>[2x]MSDLETVAKFLAESVIASTAKTSERNLRQLETQD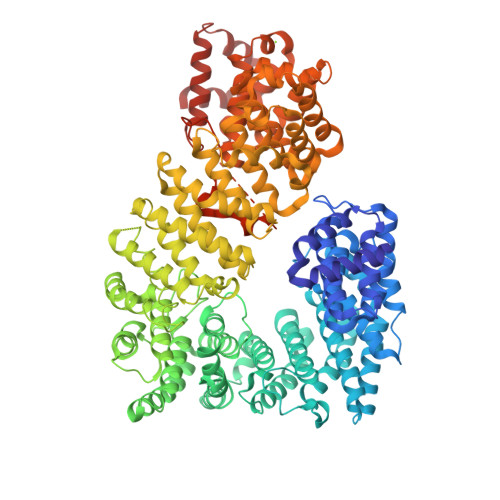GFGLTLLHVIASTNLPLSTRLAGALFFKNFIKRKWVDENGNHLLPANNVELIKKEIVPLMISLPNNLQVQIGEAISSIADSDFPDRWPTLLSDLASRLSNDDMVTNKGVLTVAHSIFKRWRPLFRSDELFLEIKLVLDVFTAPFLNLLKTVDEQITANENNKASLNILFDVLLVLIKLYYDFNCQDIPEFFEDNIQVGMGIFHKYLSYSNPLLEDPDETEHASVLIKVKSSIQELVQLYTTRYEDVFGPMINEFIQITWNLLTSISNQPKYDILVSKSLSFLTAVTRIPKYFEIFNNESAMNNITEQIILPNVTLREEDVELFEDDPIEYIRRDLEGSDTDTRRRACTDFLKELKEKNEVLVTNIFLAHMKGFVDQYMSDPSKNWKFKDLYIYLFTALAINGNITNAGVSSTNNLLNVVDFFTKEIAPDLTSNNIPHIILRVDAIKYIYTFRNQLTKAQLIELMPILATFLQTDEYVVYTYAAITIEKILTIRESNTSPAFIFHKEDISNSTEILLKNLIALILKHGSSPEKLAENEFLMRSIFRVLQTSEDSIQPLFPQLLAQFIEIVTIMAKNPSNPRFTHYTFESIGAILNYTQRQNLPLLVDSMMPTFLTVFSEDIQEFIPYVFQIIAFVVEQSATIPESIKPLAQPLLAPNVWELKGNIPAVTRLLKSFIKTDSSIFPDLVPVLGIFQRLIASKAYEVHGFDLLEHIMLLIDMNRLRPYIKQIAVLLLQRLQNSKTERYVKKLTVFFGLISNKLGSDFLIHFIDEVQDGLFQQIWGNFIITTLPTIGNLLDRKIALIGVLNMVINGQFFQSKYPTLISSTMNSIIETASSQSIANLKNDYVDLDNLEEISTFGSHFSKLVSISEKPFDPLPEIDVNNGVRLYVAEALNKYNAISGNTFLNTILPQLTQENQVKLNQLLVGNRSHHHHHH> RGSHGGSMGTEMVMVDEIPFPPQITTAKPLCLLGYGITDIEIHFLQIKFTAIGVYLEPEIVGHLQPWKGKSGKELAENDDFFEALISAPGEKFLRIVVIKEIKGSQYGVQLESAVRDRLAADDKYEEEEEEALEKVVEFFQSKYFKKDSIITFHFPATSFTAEIVFATEGKEESKITVENANVVEMIKKWYLGGTRGVSPTTISALANTLA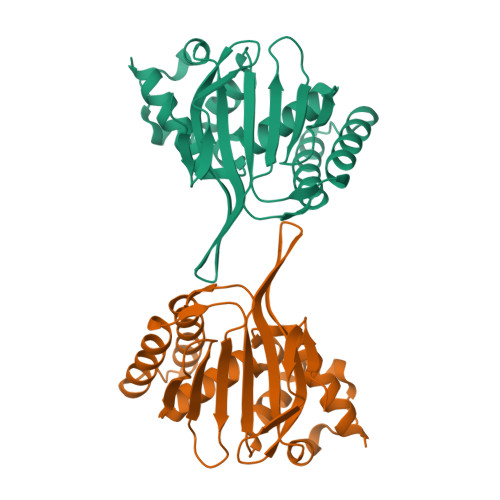TELSK> MQPYWAAIEADIERYLKKSITIRPPETVFGPMHHLTFAAPATAASTLCLAACELVGGDRSQAMAAAAAIHLVHAAAYVHEHLPPAIQHKYGPNVELLTGDGIVPFGFELLAGSVDPARTDDPDRILRVIIEISRAGGPEGMISGLHREEEIVDGNTSLDFIEYVCKKKYGEMHACGAACGAILGGAAEEEIQKLRNFGLYQGTLRGMMEMKNSHQLIDENIIGKLKELA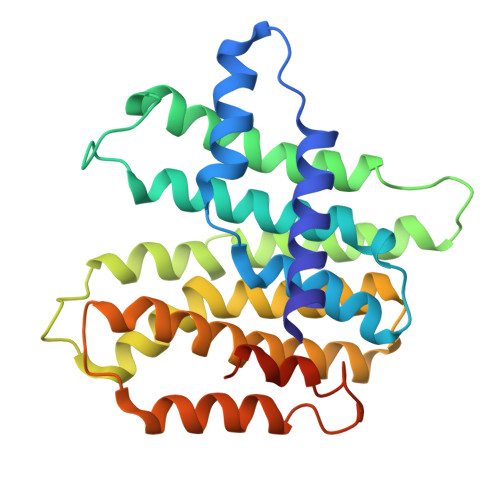LEELGGFHGKNAELMSSLVAEPSLYAAHHHHHHHH>[2x]MSKEYHIDEEVGFALPNPQENLPDFYNDWMFIAKHLPDLIESGQLRERVEKLNMLSIDHLTDHKSQRLARLVLGCITMAYVWGKGHGDVRKVLPRNIAVPYCQLSKKLELPPILVYADCVLANWKKKDPNKPLTYENMDVLFSFRDGDCSKGFFLVSLLVEIAAASAIKVIPTVFKAMQM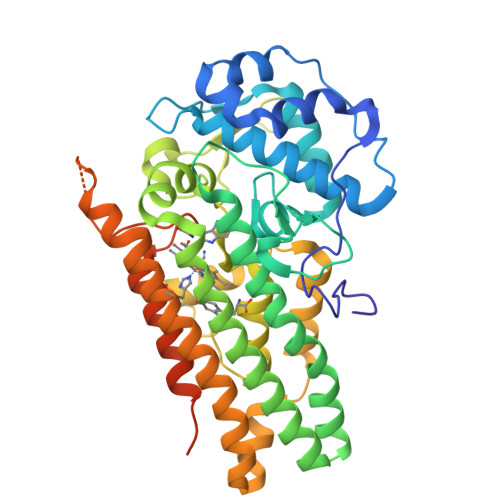QERDTLLKALLEIASCLEKALQVFHQIHDHVNPKAFFSVLRIYLSGWKGNPQLSDGLVYEGFWEDPKEFAGGSAGQSSVGQCFDVLLGIQQTAGGGHAAQFLQDMRRYMPPAHRNFLCSLESNPSVREFVLSKGDAGLREAYDACVKALVSLRSYHLQIVTKYILIPASQQPKENKTSEDPSKLEAKGTGGTDLMNFLKTVRSTTEKSLLKEGKGELNSKLEGKPIPNPLLGLDSTRTGHHHHHH> SGVDDDMACHKIPVEADFLYAYSTAPGYYSWRNSKDGSWFIQSLCAMLKQY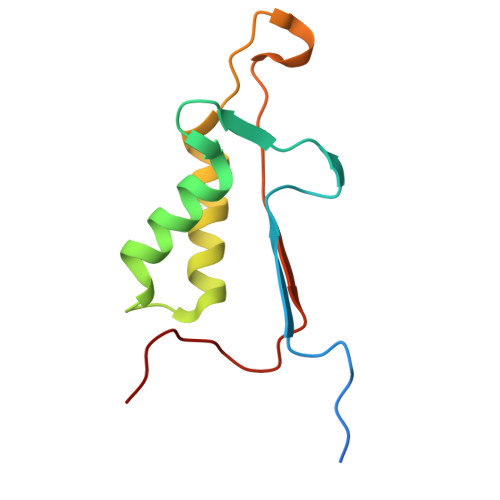ADKLEFMHILTRVNRKVADEFESFSFDATFHAKKQIPCIVSMLTKELYFYHH> MSAIKPDMKIKLRMEGNVNGHHFVIDGDGTGKPFEGKQSMDLEVKEGGPLPFAFDILTTAFLYGNR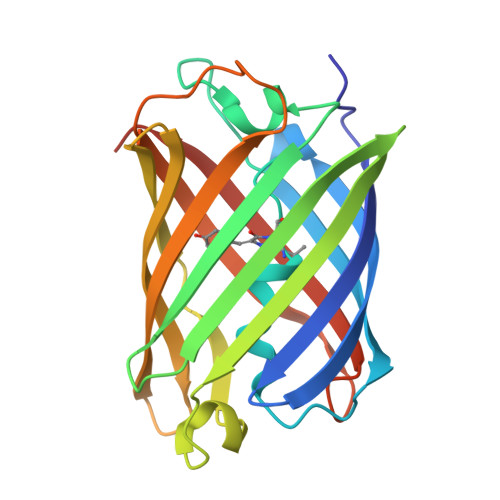VFAKYPDNIQDYFKQSFPKGYSWERSLTFEDGGICIARNDITMEGDTFYNKVRFYGTNFPANGPVMQKKTLKWEPSTEKMYVRDGVLTGDVEMALLLEGNAHYRCDFRTTYKAKEKGVKLPGAHFVDHCIEILSHDKDYNKVKLYEHAVAHSGLPDNARR> MDNKTRFMQLYEQIKNPNNGYFSPEGIPYHSVETLICEAPDYGHMTTSEAYSYWLWLEAMYGRYTQDWSKLEAAWDNMEKYIIPVNEGDNNEEQPTMNYYNPSSPATYAAEHPYPDLYPSALTGQYPAGNDPLDAELKATYGSNETYLMHWLLDVDN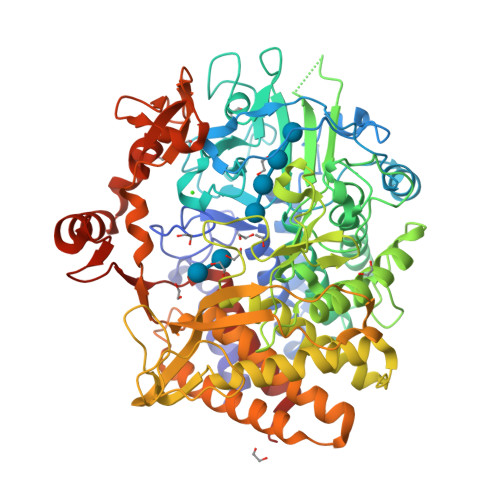WYGFGNLLNPSHTAVYVNTYQRGEQESVWETVPHPSQDNQTFGKPNEGFMSLFTKENQAPAPQWRYTNATDADARAVQAMFWARQWGYSNTNYLEKAKKMGDFLRYGMYDKYFQEIGSAADGSPSRGAGKNACHYLMAWYTAWGGGLGQYANWAWRIGASHVHQGYQNPVASYALSTAEGGLIPNSSTARSDWEKALKRQLELYTWLLSSEGAVAGGATNSWNGNYSAYPQNVSTFYEMAYTEAPVYHDPPSNNWFGMQVWPLERVAELYYIFAEKGDKSSESFHMAKHVIEKWIAYSLDYVFVGERPVTDEEGYYLNDAGERVLGGQNPQIAVQSDPGEFWIPANLEWSGQPDPWKGFDSFTGNPGLHVTTKNPSQDVGVLGSYIKTLVFFAAGTKAETGGFTALGNKAKNLAKELLDAAWSKNDGIGIAAEEEHEDYIRYFTKEIYFPNGWSGRNGQGNTIPGPNTVPSDPAKGGNGVYISHAELRPKIKNDPMWPYLENKYQTSWNPNTGKWENGLPTFVYHRFWSQVDMATAYAEYDRLIGNA In the cytoplasm, the exosome is involved in the canonical turnover of mRNA and in mRNA quality control; in the nucleus the complex degrades and processes a wide variety of RNA substrates. The exosome is a modular molecular machine that consists of an inert, nonameric core (Exo9; 300 kDa). Rrp41 and Rrp45 recruit the catalytic subunit Rrp4418 to assemble the catalytically active decameric complex (Exo10; 410 kDa). Isolated exosomes degrade single-stranded RNA irrespective of the nucleotide composition.

We determined the structure of Exo9 from the eukaryotic thermophile C. thermophilum (ctExo9) by X-ray crystallography to 3.8 Å resolution and by cryo-EM to 3.2 Å resolution. The general architecture of ctExo9 is identical to that of yeast and human exosome complexes. Despite this wealth of structural information, several disordered regions are invisible in these structures. In particular, an extended loop region in Rrp42 (Rrp42-EL) and the entry loop in Rrp41 are largely unresolved, while the shorter exit loop of Rrp41 is only partially visible. To initiate the MD simulations of the open state, all missing loops of the here obtained cryo-EM structure were modeled using the ColabFold implementation of AlphaFold2. The closed state was obtained by interactively modeling Rrp42-EL into the unoccupied cavity near Rrp41, a location that agrees with our NMR data. Finally, an analysis of the RNA channel within the representative MD simulation structures illustrates that the closed conformation of Rrp42-EL blocks the exit site of the RNA channel in the exosome core, whereas the RNA exit channel is unobstructed in the open state. The global analysis of dynamics and PRE data revealed that in Exo9 the invisible Rrp42-EL adopts the closed (open) conformation to 5 ± 1% (95 ± 1%) and that the open to closed transition takes place at a rate (kex=kopen→closed+kclosed→open) of 5800 ± 1400 s-1. The order parameter (S2) of the open conformation (~ 0.1) is significantly lower than of the closed conformation (~ 0.7), revealing that the loop in the open state is highly flexible, whereas it is stably fixed to the rest of the exosome complex in the closed state. Rrp42 in C. thermophilum thus contains a previously unidentified flexible one-way-plug that readily allows for passage of substrate RNA via the through-channel route but that prevents access to the Rrp44 active site via an aberrant direct path.

> MPREVEPSLSERQFVLQALQEGLRLDGRQLDQYRPLSLTFGDQYGVADVTFGKTRVLAKASAEVTVPYADRPLDGIFTIATELSPMTSPTFEVNRPTETEVLLSRLLEKTIRRSGALDTESLCLVAGQKCWSIRVDVHVMSHDGNLVDAACIAVVAALRHFRKPDTSIESGVLTIYTPAEREPVPLSWLHTPFCVTWSFFGDEGEIAVLDATWLEEQVRVGSCTISMNKHGEICQIAKLGGTPVEAVSLLQCTSIALTKVKEFSDLVDKKLAEDFKRRNPGGLLKELKAENDR;> MPLDTSTYKLALLRVDGRRWNELRRVHAQIRTQAAADGSSYLEMGHTKVMCVVTGPSEPGPRRGTGAGTTGGGGAGGAGGGGSGGQGKEAEVVVSIVIAGFSSVDRKRHGRNDKRIIEMQSTVANALSASLHTHLFPHSQITISLHVLSQDGSLLAALINAATLACVDAGIPMTDYVVACTAGSTSTYAANDENADPLLDLNHQEEQELPWLTVATLGESDKVAVLVCESRVQVSRLEGMLAVGVDGCKQIRAILDHVVRQKGRRMIREGAVEKGVSLDDMDED;> MATDAASAPHSLTFPRGIFAKLSPHPYLLRTLCPDPSNSSSTPQRTNGRRPNEARPFRVNLGSLSHAHGSALVRAGDTTVLCGVRGEVLPVERIPLFRQPDVNGSGIGATVGRGELKEYDLLVPNIELATGSAPQFLPGVPPTALAQTLSTRVYSLLHSTRLVSAEELRIWYRPVATNRSKEGEDVEMEEECQEESGEEQDRVVAYWVLYIDLVFLSFDGNPFDVAWAAVVAALRDTKLPVARWDPDREMVVCSKTETMKLTIKGLPIACSAAVFLEKEHGEVAVGEKNRHWILLDPDRLEESLCKEVITMVVDFSDGETRIRAIEKQGGTVFGRELIRSFALVAEDRWKVVKEVMK;> MTTTTATTAPEAALGVLPRADGSARYSHAGYTVTASVNGPIEAQRRDEHPYEAHVDVIVRPAAGVGGTRERHLESILQSSFAQIILVKSFPRSLIQIVLQVEESPENEYVNTKLVQASLNFAVMPALFQTAMLALLSAGVPMRATATATAIALASENGATKTLIDPSPRQVELAQSVHVFAFTSQDELLLAESEGDFTIKEWDAAYETAKNICCRPSPTMDGVQMMAIDDDRLVGPDLRHFIRSTMEAKVATDLHWKS;> MSAASSQHVLLSPAELAYLHASLSLTPPIRPDGRSPTQFRPLIAETGILPGANGSARVCFADGTEAIVGVKAEVEKTVSRSKEDEEVGLLVASAGDMDVDDEEGYAKVGADNRTGEASWVEITVEIPGVRDDDSGMVFLAQLLGEALLADGEFVKKLWINRRYHWKLYIDILLISPPLSYPLPLLSLTTHLALLSTRLPRLKSEGDEDPYFDDDWAVAPYLFPRSSSASKSSKSSPTQPTTRPPITLLVMAVGNNILFDPSKEELAVADVALAVSVTATDVDPDESDAQKETATATAGPDSADAAKRGRKLRLLSIRTIDPPSRLTPPGVPNSTNPAAIYGTTSSSGTNGNGQPQQKVESGKISEPIEPIEGVWRAPRGGAKRLVLGALVQKVLEKGGVVDEVLDALEGVELT;> MTDRRRINGPAGATIPPVYEDSGISEVKALKIRSRPSNIIRKIYLKTGVTPSASGSAYLELETSANSGVSGLKLSCTVHGPRSLPRSSPFSPHMVVSTHVKYAPFATKQRRGYLRDPTERDLGIHLEAALRGAIIADRWPKSGVDIIISIIEGDQDREASKTQGDEVWDMMNTLSGCITVASAALADAGIDCVDTVAGGVAALVQDSDGSPEIVVDPIPSEHRKILAACCVAYLPMRDEVTNLWFRGDLPASDMDLYTELVEKGIQASRSANRVLVDCLTETVG;> MSTTTRPFVLPGETIDPSLVPTHPKHPLRLGPGLRHVPPSDIIPTVAGQLITNLNKNSMWVEYNSQRYVPTQNDLVLAQVLRSTQDSYLCLITPHTPPATLPHLAFESATKKTRPQLQPGQLVYARVSLANRHMDPELECVNPSTGKADGLGPITGPGCVFEVSLGFARRLLMAKSREEGKVGVLEMLAGEDPSIGEAGAGLAFETAVGRNGRVWVGSEDVKTVIIVGRALQETDRGNLTIEGQRKLVRRLLREMR;> MPITIHAPLPPPRLHDEDSDVDMSSDSDSSSEGGVPLTSNLPSRAKPKSSLFTTTKSSSDIVTPGELITTSPQFMRGHGTYIPPGTTSIISSVAGTILRTNKLLSVRPLRARYTPEVGDLVVGRIIEVQARRWRVDVGSTQFASLPLSAINLPGGILRKRTETDELQMRSFFSEGDLLVAEVQGVYGDGGAVLHTRSLKYGKLRNGVFVAVSGMGGGGGVVRSRRQVWTLEGANGAGLIDVVLGVNGYVWIAKHTEDGPGEDPNASTKQVGITNLEEGMSANMYSSQNDRIEAETMREIARLRGVVMALVENGLRVDEDMVMRGYREAVEMALVSPEGPEDVYLGGERGRQLAAALTA;> MTTTQPTLALPGQLLGPISKYQPGPGTHVHESNLYSSLLGTVHVTQPARAPGPVKRLNRITPAPTPAELPTISVSAARPAGSAASGLVTGRKREILPEVGNIVLCRVIRITPRQAVVTILVCGDTVLDAEWQGLIRVQDIRATEKDRVKVYESFRPGDIVRAEVISLGDQANYYLSTARNELGVILATSEAGNTMYPVSWREYRDPITGLTELRKVAKPY> GSPGILAPLAPGSEDNFARFVCKNNGVLFENQLLQIGLKSEFRQNLGRMFIFYGNKTSTQFLNFTPTLICADDLQTNLNLQTKPVDPTVDGGAQVQQVINIECISDFTEAPVLNIQFRYGGTFQNVSVKLPITLNKFFQPTEMASQDFFQRWKQLSNPQQEVQNIFKAKHPMDTEITKAKIIGFGSALLEEVDPNPANFVGAGIIHTKTTQIGCLLRLEPNLQAQMYRLTLRTSKDTVSQRLCELLSE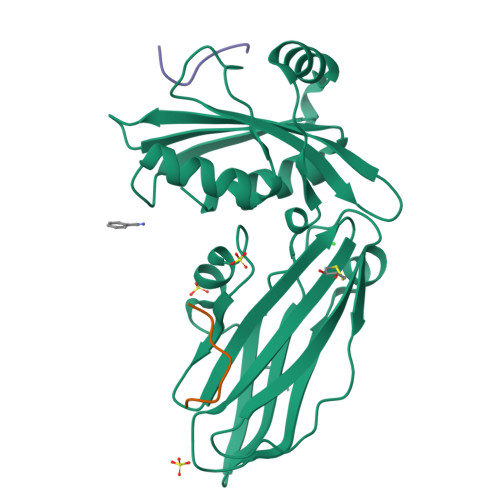QF;> NPKGWVTFEEEE;> FEDNFVP>GAMDPQFMKKVAVIDIEGTLTDFEFWREMARITGKREIEELLEKGLSGEVEWLDSLLKRVGLIRGIDEGTFLRTREKVNVSPEARE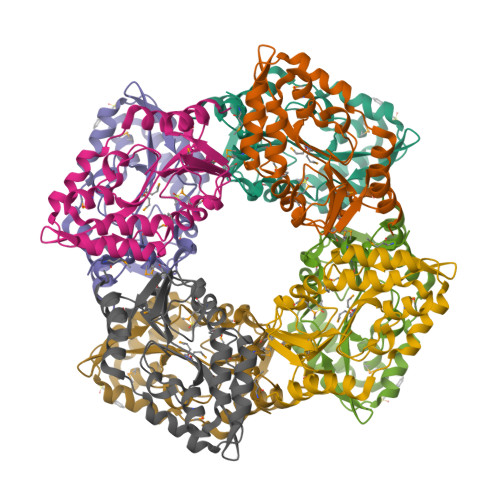LVETLREKGFKVVLISGSFEEVLEPFKELGDEFMANRAIFEDGKFQGIRLRFRDKGEFLKRFRDGFILAMGDGYADAKMFERADMGIAVGREIPGADLLVKDLKELVDFIKNLKP[4x]> GKELEIVARLQQLNIELARKLLEAVARLQELNIDLVRKTSELTDEKTIREEIRKVKEESKRIVEEAEQEIRKAEAESLRLTAEAAADAARKAALRMGDERVRRLAAELVRLAQEAAEEATRDPNSSDQNEALRLIILAIEAAVRALDKAIEKGDPEDRERAREMVRAAVRAAELVQRYPSASAANEALKALVAAIDEGDKDAARCAEELVEQAEEALRKKNPEEARAVYEAARDVLEALQRLEEAKRRGDEEERREAEERLRQACERARKKN

We develop a hierarchical approach to designing multi-component protein assemblies from two classes of modular building blocks: designed helical repeat proteins (DHRs) and helical bundle oligomers (HBs). We first rigidly fuse DHRs to HBs to generate a large library of oligomeric building blocks. We then generate assemblies with cyclic, dihedral, and point group symmetries from these building blocks using architecture guided rigid helical fusion with new software named WORMS. X-ray crystallography and cryo-electron microscopy characterization show that the hierarchical design approach can accurately generate a wide range of assemblies, including a 43 nm diameter icosahedral nanocage.

To build such structures by helix fusion using our building blocks with smaller and weaker interfaces that give rise to cooperative assembly, we systematically split each DHR at the loop in the center of four repeats, resulting in a hetero-dimeric structure with two repeats on each side. Tetrahedral, octahedral, and icosahedral assemblies were generated from C5, C3, and C2 building blocks placed on their respective point group symmetry axes, connected by the split DHRs heterodimers. Following fusion, sequence design was performed at each of the two new junctions. For another design, T32_Wm-24, while the full cage did not assemble, we were able to crystallize the polar-capped trimer component (C3_HF_Wm-0024A) and solve the structure by X-ray diffraction to 2.69 Å. The structure clearly shows that both of the newly designed junctions (from HF and WORMS) are as designed, matching the design model.> NIVFDVENATPETYSNFLTSLREAVKDKKLTCHGMIMATTLTEQPKYVLVDLKFGSGTFTLAIRRGNLYLEGYSDIYNGKCRYRIFKDSESDAQET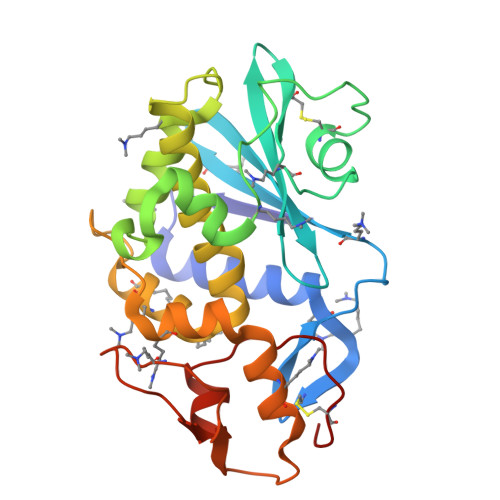VCPGDKSKPGTQNNIPYEKSYKGMESKGGARTKLGLGKITLKSRMGKIYGKDATDQKQYQKNEAEFLLIAVQMVTEASRFKYIENKVKAKFDDANGYQPDPKAISLEKNWDSVSKVIAKVGTSGDSTVTLPGDLKDENNKPWTTATMNDLKNDIMALLTHVTCKVK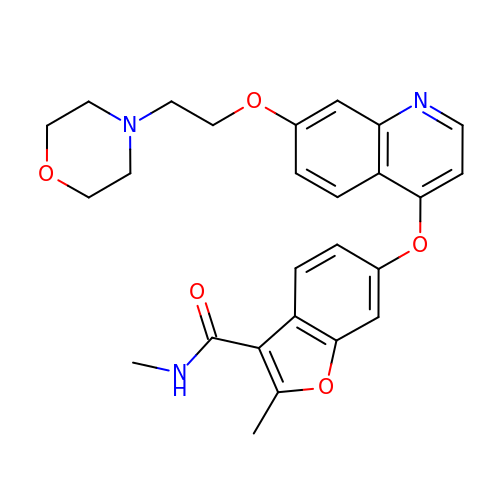N,2-DIMETHYL-6-{[7-(2-MORPHOLIN-4-YLETHOXY)QUINOLIN-4-YL]OXY}-1-BENZOFURAN-3-CARBOXAMIDE | C26 H27 N3 O5 | LGXVKMDGSIWEHL-UHFFFAOYSA-N>MAELPPGRLATTEDYFAQQAKQAVTPDVMAQLAYMNYIDFISPFYSRGCSFEAWELKHTPQRVIKYSIAFYAYGLASVALIDPKLRALAGHDLDIAVSKMKCKRVWGDWEEDGFGTDPI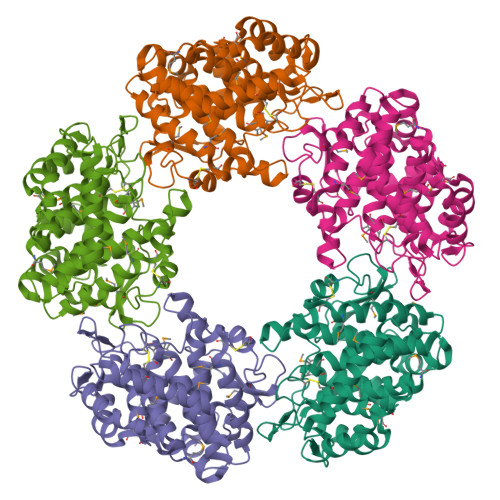EKENIMYKGHLNLMYGLYQLVTGSRRYEAEHAHLTRIIHDEIAANPFAGIVCEPDNYFVQCNSVAYLSLWVYDRLHGTDYRAATRAWLDFIQKDLIDPERGAFYLSYHPESGAVKPWISAYTTAWTLAMVHGMDPAFSERYYPRFKQTFVEVYDEGRKARVRETAGTDDADGGVGLASAFTLLLAREMGDQQLFDQLLNHLEPPAKPSIVSASLRYEHPGSLLFDELLFLAKVHAGFGALLRMPPPAAKLAGK[5x]>GAMSEAFHTHSGIGVPLRRSNVDTDQIIPAVFLKRVTRTGFEDGLFAGWRSDPAFVLNLSPFDRGSVLVAGPDFGTGSSREHAVWALMDYGFRVVISSRFGDIFRGNAGKAGLLAAEVAQDDVELLWKLIEQSPGLEITANLQDR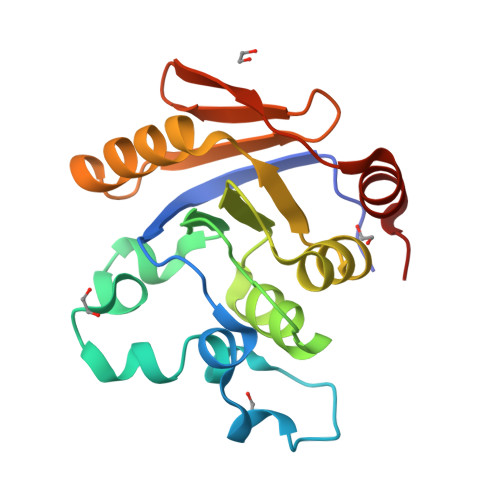IITAATVVLPFKIDDHSAWRLLEGLD[2x]> RAPDSVDYRKKGYVTPVKNQGQCGSCWAFSSVGALEGQLKKKTGKLLNLSPQNLVDCVSENDGCGGGYMTNAFQYVQKNRGIDSEDAYPYVGQEESCMYNPTGKAAKCRGYREIPEGNEKALKRA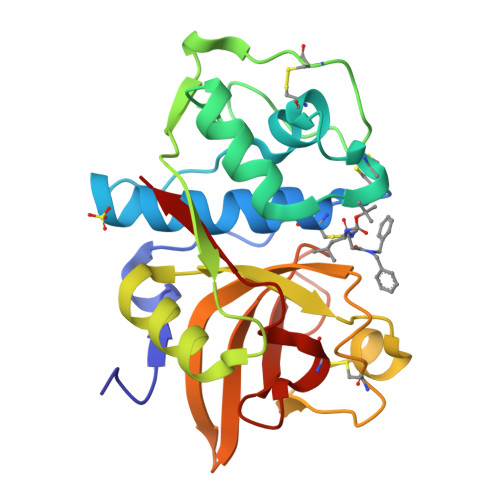VARVGPVSVAIDASLTSFQFYSKGVYYDESCNSDNLNHAVLAVGYGIQKGNKHWIIKNSWGENWGNKGYILMARNKNNACGIANLASFPKM> TEKKYIVALDQGTTSSRAVVMDHDANIISVSQREFEQIYPKPGWVEHDPMEIWATQSSTLVEVLAKADISSDQIAAIGITNQRETTIVWEKETGKPIYNAIVWQCRRTAEICEHLKRDGLEDYIRSNTGLVIDPYFSGT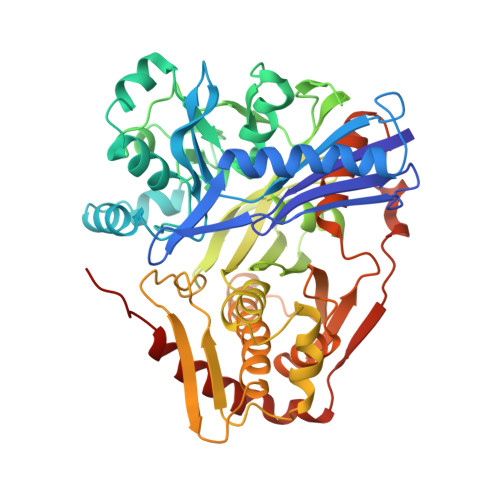KVKWILDHVEGSRERARRGELLFGTVDTWLIWKMTQGRVHVTDYTNASRTMLFNIHTLDWDDKMLEVLDIPREMLPEVRRSSEVYGQTNIGGKGGTRIPISGIAGDQQAALFGQLCVKEGMAKNTYGTGCFMLMNTGEKAVKSENGLLTTIACGPTGEVNYALEGAVFMAGASIQWLRDEMKLINDAYDSEYFATKVQNTNGVYVVPAFTGLGAPYWDPYARGAIFGLTRGVNANHIIRATLESIAYQTRDVLEAMQADSGIRLHALRVDGGAVANNFLMQFQSDILGTRVERPEVREVTALGAAYLAGLAVGFWQNLDELQEKAVIEREFRPGIETTERNYRYAGWKKAVKRAMAWEEHDE5-[(1S)-1-(4-methoxyphenyl)ethyl]-1',3'-dimethyl-1'H,2H-3,4'-bipyrazole | C17 H20 N4 O | 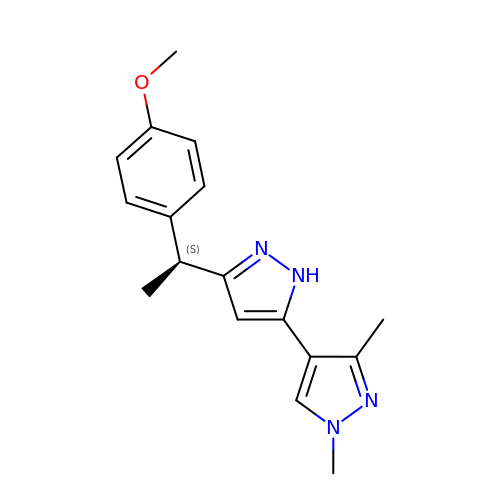MWUFWVBVAVNBCP-NSHDSACASA-N>[4x]MKAAVLHEFGQSLQIEEVDIPTPGAGEIVVKMQASGVCHTDLHAVEGDWPVKPSPPFIPGHEGVGLITAVGEGVTHVKEGDRVGVAWLYSACGHCTHCLGGWETLCESQQNSGYSVNGSFAEYVLANANYVGIIPESVDSIEIAPVLCAGVT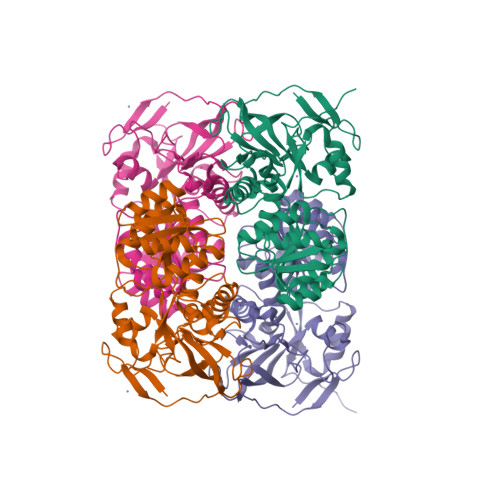VYKGLKMTDTKPGDWVVISGIGGLGHMAVQYAIAMGLNVAAVDIDDDKLAFAKKLGAKVTVNAKNTDPAEYLQKEIGGAHGALVTAVSAKAFDQALSMLRRGGTLVCNGLPPGDFPVSIFDTVLNGITIRGSIVGTRLDLQESLDMAAAGKVKATVTAEPLENINDIFERMRQGKIEGRIVIDYTMLEHHHHHH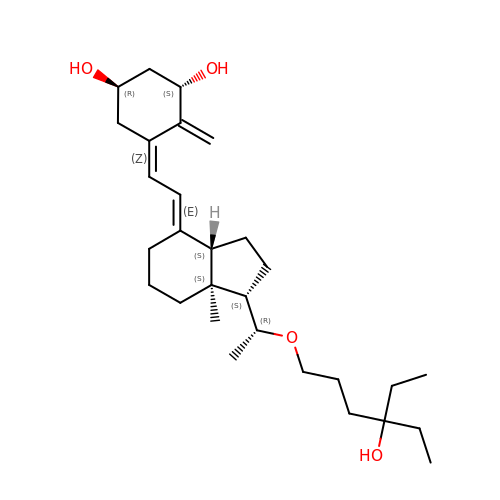5-(2-{1-[1-(4-ETHYL-4-HYDROXY-HEXYLOXY)-ETHYL]-7A-METHYL-OCTAHYDRO-INDEN-4-YLIDENE}-ETHYLIDENE)-4-METHYLENE-CYCLOHEXANE-1,3-DIOL | C29 H48 O4 | KLZOTDOJMRMLDX-YBBVPDDNSA-N>MVRFLDGHTPAYDLTYNDVFVVPGRSDVASRFDVDLSTVDGSGTTIPVVVANMTAVAGRRMAETVARRGGIVVLPQDLPITAVSETVDFVKSRDLVVDTPVTLSPEDSVSDANALLHKRAHGAAVVVFEGRPIGLVTEANCAGVDRFARVRDIALSDFVTAPVGTDPREVFDLLEHAPIDVAVMTAPDGTLAGVLTRTGAIRAGIYTPAVDAKGRLRIAAAVGINGDVGAKAQALAEAGADLLVIDTAHGHQAKMLDAIKAVASLDLGLPLVAGNVVSAEGTRDLIEAGASIVKVG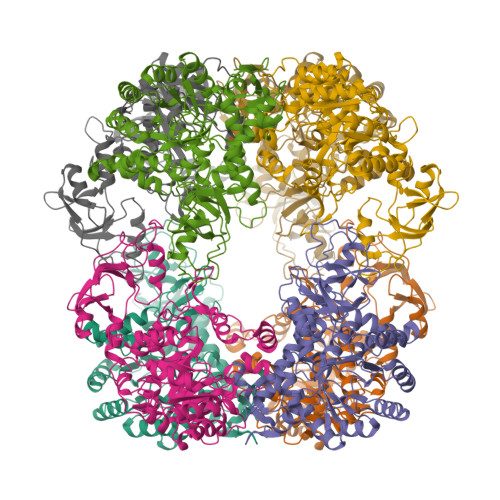VGPGAMCTTRMMTGVGRPQFSAVVECAAAARQLGGHVWADGGVRHPRDVALALAAGASNVMIGSWFAGTYESPGDLLFDRDDRPYKESYGMASKRAVAARTAGDSSFDRARKGLFEEGISTSRMSLDPARGGVEDLLDHITSGVRSTCTYVGAANLPELHEKVVLGVQSAAGFAEGHPLPAGWTAAAKEDLEHHHHHHHH[8x]> GHMASVNAETVAPEFIVKVRKKLSLTQKEASEIFGGGVNAFSRYEKGNAQPHPSTIKLL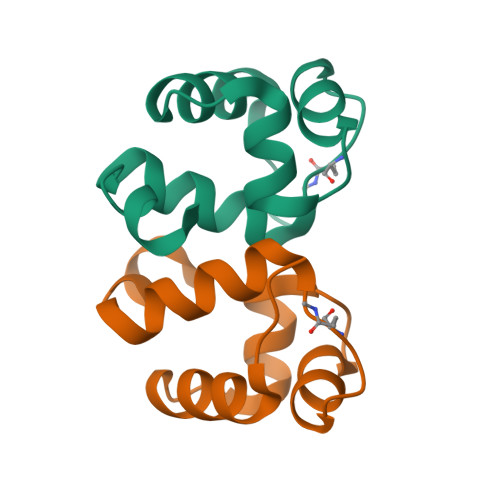RVLDKHPELLNEIR> DEDKDKDETE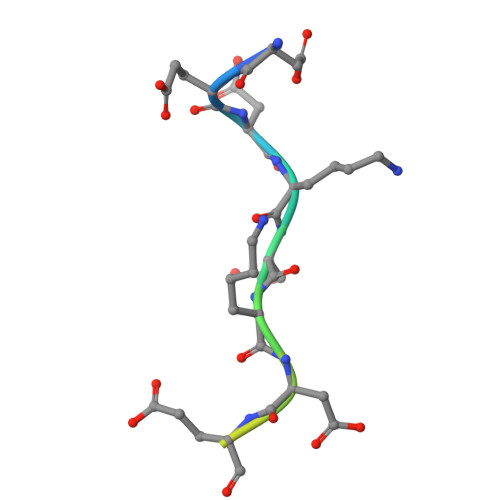TVKQT> HRXV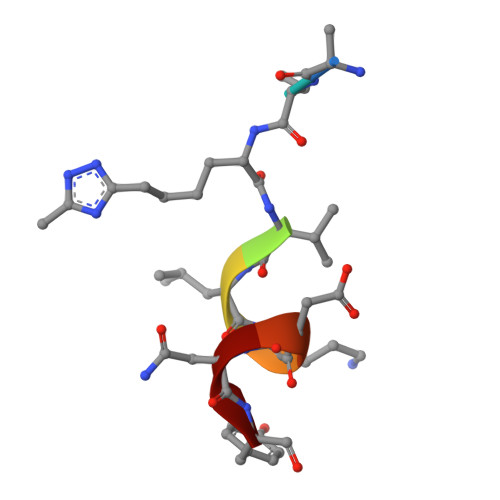LRDNY> MQNSQEMAITTLSLPKGGGAINGMGESVGQAGPDGMVTFSIPLPFSAGRGVAPALSLSYSSGAGNGPFGMGWQCSAMSISRRTQKGVPQYNEDDEFLSPSGEVMAIALNDSGFEDVRTANRLQGIPLPFSYKVTRYQPRLIQDFIKIEYWQPVKQTDGTPFWIIYSPDGQTHILGKNSHSRVANAENPSQIASWLLEETVTPTGEHIYYQYSGENQVNCTDAEIALHPQDSAQRYLARIDYGNISPQASLFVLDEELPNLTQWLFHLVFDYGERDISINKIPTFEGGTTGWLARPDMFSRYDFGIEIRNRRLCHQVLGFHRLEALNDRDVTDEIPVLVNRLTLDYDLNNSVSTLVAVRQVAYETDGSPITQPPLEFDYQRFDTGSIPGWQEMPQLEAFNGYQPYQMIDLYGEGTPGILYQETPGAWWYKSPQRQIGGDSNAVTYGAMKALPKIPRLQEGATLMDINGDGRLDWVITSAGVRGFHSIHSTGEWTHFTPLNTLPTEYFHPKAQLADLVGAGLSDLVLIGPKSVRLYANQQGNWAPAQDVTQAENVSLPVIGIDSRQLVAFADMLGSGQQHLVEITADSVKCWPNMGHGRFGQPLTLEGFSQPQTSFNPDRVFLADIDGSGTNDIIYAHSECLEIYLNESGNRFSKPISLLLPDGVNFDNTCQLQAADIQGLGIASLVMTVPHMSPTHWRCDLALNKPWLLNVMNNNRGAETCLFYRSSAQFWLDEKQLVEAAGQQPECHLPFPMHLHWRSEIFDEITGNRLTQEQEYAHGSWDGQEREFRGFGRLIQRDTDGFAQGTVDIPTHPSRTVSWFATGIPEIDTTLSAEFWRGDDQAFSPFSPRFTRWENDSEAGSDVAFIPSEHDAFWLNRAMKGQLLRSELYGDDGTPEAEIPYSVTEMRHQVRALPTTDATVPSAWCSTIETRSYQYQRVAADPQCSQQVVIKADRYGSPLLSVAINYPRRKKPEKSPYPDDLPETLFDSSYDTQQQQLHLTKQQQNYFHLTNDDNWLLGLPKEQRNDGYQYDQERAPAN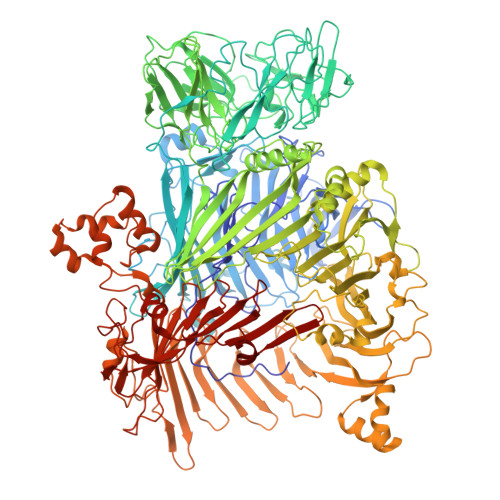GFTLETLIASNSLIGSNQPFTYLGQSRVAYQGGVDEQPSLQALVAYGETAILDEKTLQAFVGVLDSKTRDELLFSAGYQLAPRLFRVESEPDVWVARQGYSEFGDYSQFWRPLSQRSTLLTGKTTLKWDKHYCVVIETQDAAQLVTQARYDYRFLTPYSLTDANDNQHYVVLNPFGEVIASRFWGTEAGKDAGYSTPQAKPFVVPATIEAALALSPGIPVAHCAIFEPESWMQKLTQHDVSERMADNGTLWNALLQARFVTEDGYVCALGRRRWMARHGLSVLMLTLLAEIPRTPPHSLTITTDRYDSDDQQQLRQRILFSDGFGRLLQSAQRVEAGESWQRSEDSSLVVNVSGTPALVVTDNRWAVSGRTEYDGKGQGIRVYQPYFLDDWRYLSDDSARTDLFADTHIYDPLGREYQVITAKGYRRERQYTPWFVVNQDENDTAANLAI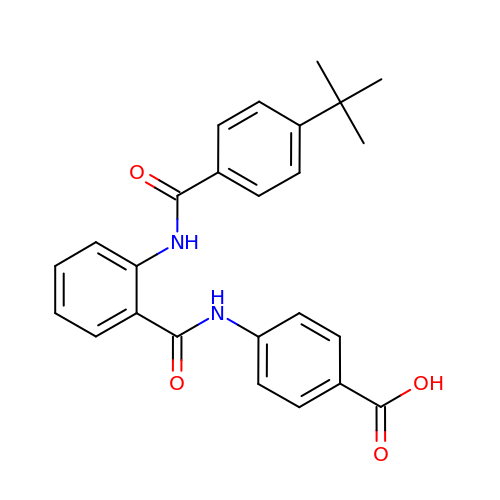4-({2-[(4-tert-butylbenzoyl)amino]benzoyl}amino)benzoic acid | C25 H24 N2 O4 | JNIQPWWGQWIPLQ-UHFFFAOYSA-N>DSTGYDKDLVEALERDIISQNPNVRWDDIADLVEAKKLLKEAVVLPMWMPEFFKGIRRPWKGVLMVGPPGTGKTLLAKAVATECKTTFFNVSSSTLTSKYRGESEKLVRLLFEMARFYSPATIFIDQIDSICSRRGTSEEHEASRRVKAELLVQMDGVGGTSENDDPSKMVMVLAATN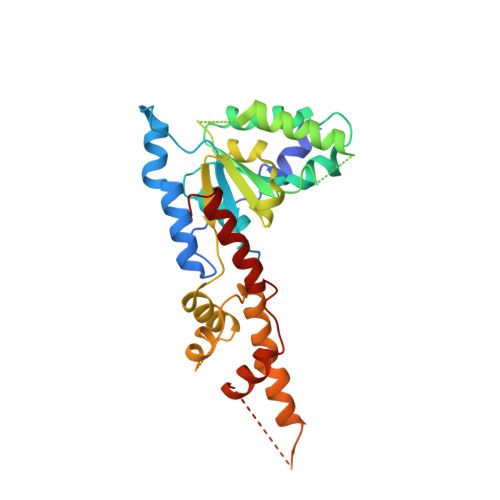FPWDIDEALRRRLEKRIYIPLPSAKGREELLRISLRELELADDVDLASIAENMEGYSGADITNVCRDASLMAMRRRIEGLTPEEIRNLSKEEMHMPTTMEDFEMALKKVSKSVSAADIERYEKWIFEFGSC[2x]>WGNLGHETVAYIAQSFVASSTESFCQNILGDDSTSYLANVATWANTYKYTDAGEFSKPYHFIDAQDNPPQSCGVDYDRDCGSAGCSISAIQNYTNILLESPNGSEALNALKFVVHIIGDIHQPLHDENLEAGGNGIDVTYDGETTNLHHIWDTNMPEEAAGGYSLSVAKTYADLLTERIKTGTYSSKKDSWTDGIDIKDPVSTSMIWAADANTYVCSTVLDDGLAYINSTDLSGEYYDKSQPVFEELIAKAGYRLAAWLDLIASQPS[2x]

S1 nuclease from Aspergillus oryzae (EC 3.1.30.1; NCBI sequence ID: XP_001818636; S1–P1 nuclease family in Pfam, PF02265) is an extracellular, single–strand–specific, sugar non–specific, Zn2+–dependent, fungal nuclease with 3'–mononucleotidase activity with a pH optimum in range 4.0–4.3. S1 nuclease has the phospholipase C/P1 nuclease–like fold stabilized by two disulfide bridges. The active site is located in a surface cleft and composed of the obligatory catalytic trinuclear zinc cluster supplemented by Lys68 and the nucleoside binding site 1 (NBS1; also called Phe site in the previous studies). A cluster of three zinc ions coordinates the substrate/product scissile phosphate and the reaction mechanism utilizes water activated by Zn2+ ions as a nucleophile.

The mutant D65N has the same tertiary structure as the wild type. The active site organization is also unchanged, with the only difference being the change of Asp65 to Asn. Products of 3’monunucleotidase activity are bound in the active site: phosphate with 2’–deoxycytidine or 2'–deoxyguanosine. A phosphate ion is bound inside the zinc cluster in the first binding mode in protein chain A. The second molecule of dCyt binds in the secondary binding site composed of Tyr183 providing a stacking interaction for the nucleobase and Glu177 providing hydrogen bonding. We refer to this site as “Half–Tyr site” with respect to the P1 nuclease Tyr site which is composed of two tyrosine residues. Chain B also contains a phosphate ion in the first binding mode. Simultaneously, one molecule of 2'–deoxyguanosine (dGua) is bound in the active site, interacting with NBS1 and the zinc cluster. In this binding mode deoxyribose is oriented out of the active site without any direct interaction with the protein.>[2x]MGHHHHHHGDPTTDDAIVAANNKFTLEYFKACYDEKCNCAVSPYHVRLALSMFYPLAGAAVQEDFQVAFGLPEDVHAAIEQQQRLAQQLHDGQHLKALSFVLVEET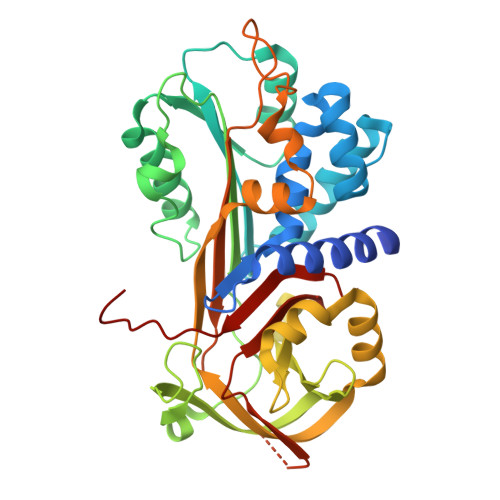LRLDSEFERLFHRTFQTTVEPVDLTDDIPSALAVNSFYQRANTEIEDFIGEGDVFSLPPCHKLMLFSGVSVLTPLAIRFNPADTALELFQFINAPTQRVSTMHTTAFVRRCLHNELRCKVVDMPFDAASGLSMLVLLPYDGTELRQIVNSITPAHLAQIDERLQSCWTDLKLPKFFVREKTDPKQTLGKLGYGGVFEIDDLHVFHDSGRTRLNGFIQHCYLAVSESGSGIPAPPDTPSEFEFHANRPFMFLIRRTMDGNVLQVGNFSKYIDPDEQF>MNLCNVNNYYLIIAEKSKAAKKIAEALSEKPILCRKYNVSYWIIKDHNSSKYVIVPAAGHLFGLKGESGFPVYDADWKPLWEIDKNSYYTKRYYQLISSLSKYALGFINACDYDIEGSVIGYLIIKNLGDIKKAKRMKFSALTKSDILSAFRNISALDYDMINAGIARHKIDWLWGINVSRALMISLQDFAKKRVILSAGRVQSPTLVQVVNSEIERNLFIPLPKFTVSIIVKIKDYSLNIKVNKEFEKITEAKEFLNKLINKTVKVVEVENRVRLLERPSPFNLTDLQIEAGRIYGISPYNVERIAEDLYLDGLISFPRTNSQKIPSTISIYNIIKGLENSSYRKLVDLVRKITGGKYVVKQGIKDDPAHPAIHPTGEAPKNLPNSKFKIYDLIARRFLGSVSADAKLSNTIYTLKVSDFPLEFTVSYTKILERNWLDIYHFHNVKEDKPIFLSKGDEGKIVDGKVNISLSKPTSRYTKVSLLKWMESSNLGTEATRGRIIEILVKRKYLTNNGRYIIPTKLGFYIAEILNKFFPDIVDVRMTADMESKLEMIKTGKVLESKVIKENIEKLNKF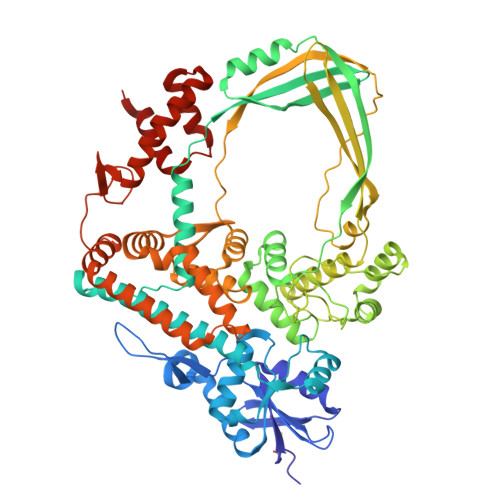IEEYKVNKDKVGESLAKALGLIKIVKCKYCDLEQYKDGLCKYHYEAKVRLLDAVEIWKERTKYDHKKILKRISSSKSTGKYVKDIVTYMLSSE[4x]> GSSGSSGGTTCPPPVSI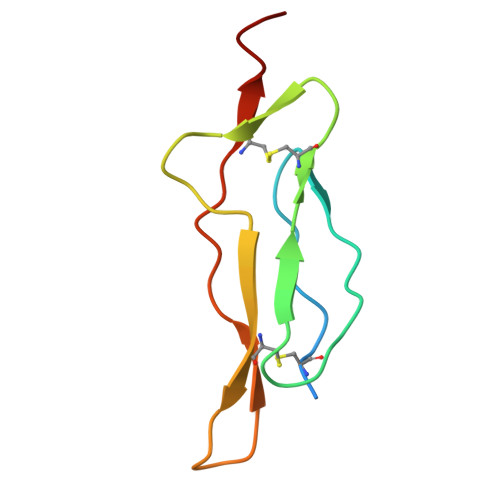EHADIRVKNYSVNSRERYVCNSGFKRKAGTSTLIECVINKNTNVAHWTTPSLKCIRDPSLA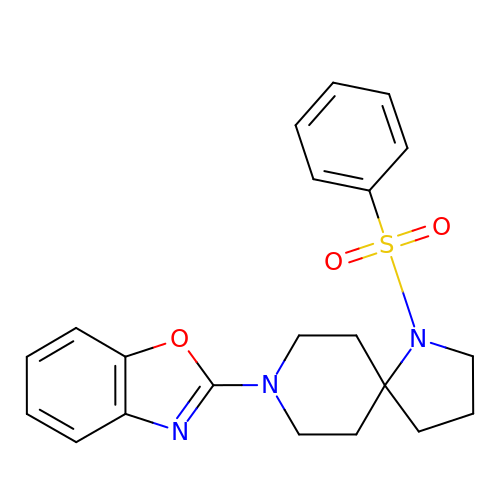2-[1-(phenylsulfonyl)-1,8-diazaspiro[4.5]decan-8-yl]-1,3-benzoxazole | C21 H23 N3 O3 S | KIKWLYIDCILHAP-UHFFFAOYSA-N> ARSEKRVPMTRLRKRVAERLLEAKNSTAMLTTFNEVNMKPIMDLRKQYGEAFEKRHGIRLGFMSFYVKAVVEALKRYPEVNASIDGDDVVYHNYFDVSMAVSTPRGLVTPVL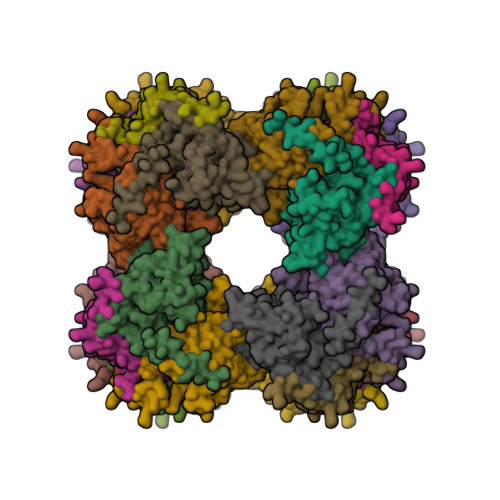RDVDTLGMADIEKKIKELAVKGRDGKLTVEDLTGGNFTITNGGVFGSLMSTPIINPPQSAILGMHAIKDRPMAVNGQVEILPMMYLALSYDHRLIDGRESVGFLVTIKELLEDPTRLLLDV> KMSDVKCTSVVLLSVLQQLRVESSSKLWAQCVQLHNDILLAKDTTEAFEKMVSLLSVLLSM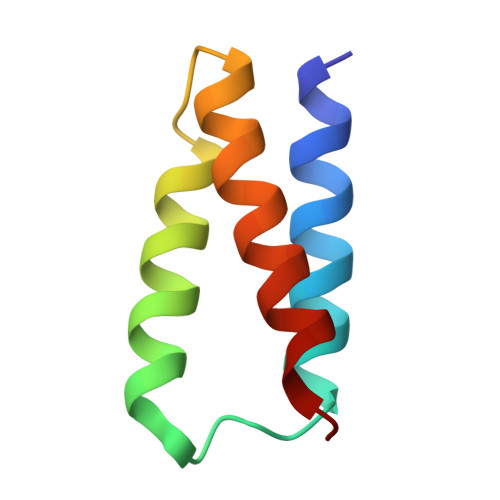QG> KSCPNPGEIRNGQIDVPGGILFGATISFSCNTGYKLFGSTSSF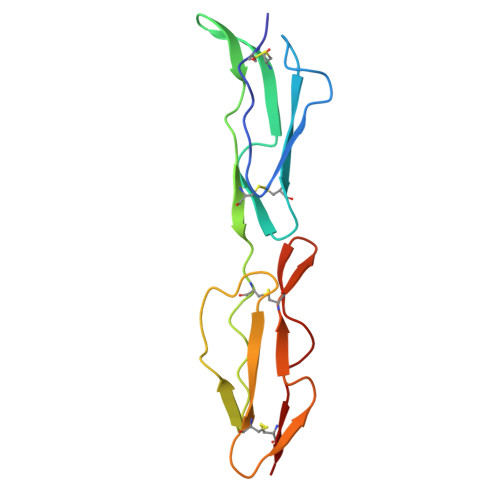CLISGSSVQWSDPLPECREIYCPAPPQIDNGIIQGERDHYGYRQSVTYACNKGFTMIGEHSIYCTVNNDEGEWSGPPPECRG N-(3-cyano-4,5,6,7-tetrahydro-1-benzothien-2-yl)-2-fluorobenzamide | C16 H13 F N2 O S | 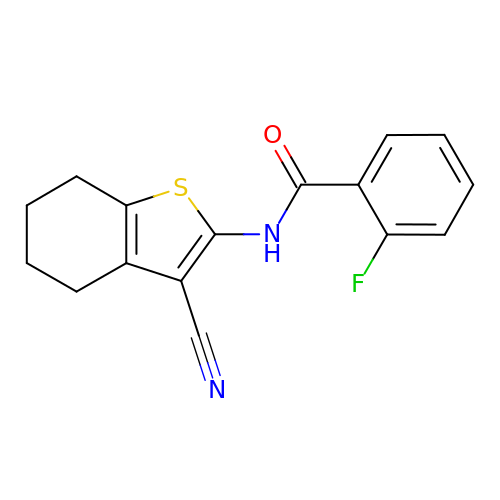YVYPYORTKAIUGJ-UHFFFAOYSA-N>YSGPKLEDGKVTISFMKELMQWYKDQKKLHRKCAYQILVQVKEVLSKLSTLVETTLKETEKITVCGDTHGQFYDLLNIFELNGLPSETNPYIFNGDFVDRGSF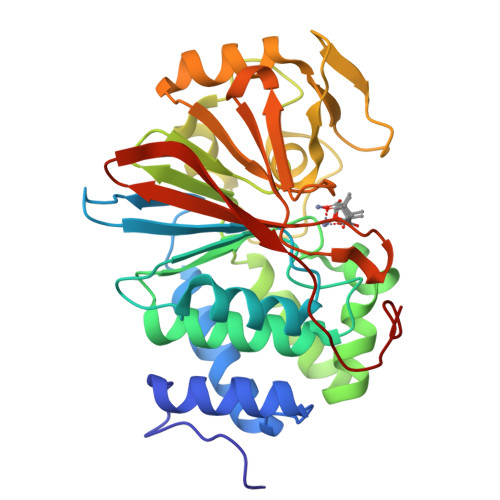SVEVILTLFGFKLLYPDHFHLLRGNHETDNMNQIYGFEGEVKAKYTAQMYELFSEVFEWLPLAQCINGKVLIMHGGLFSEDGVTLDDIRKIERNRQPPDSGPMCDLLWSDPQPQNGRSISKRGVSCQFGPDVTKAFLEENNLDYIIRSHEVKAEGYEVAHGGRCVTVFSAPNYCDQMGNKASYIHLQGSDLRPQFHQFTAVPHPNVKPMAYA[2x]> MLRVAYEGSDSEKGEGAEPLKVPVWEPQDWQQQLVNIRAMRNKKDAPTTELNFSSPKVRRYQVLLSLMLSSQTKDQVTAGAMQRLRARGLTVDSILQTDDATLGKLIYPVGFWRSKVKYIKQTSAILQQHYGGDIPASVAELVALPGVGPKMAHLAMAVAWGTVSGIAVDTHVHRIANRLRWTKKATKSPEETRAALEEWLPRELWHEINGLLVGFGQQTCLPVHPRCHACLNQALCPAAQGLEHHHHH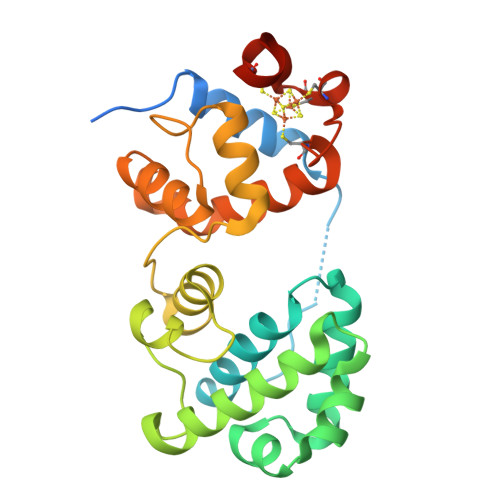H> MKGTYLYLNIYKRKREASLITLNYIKNRFYPSKIQKIIKELFEDRLKGVEYDPNNANQLSE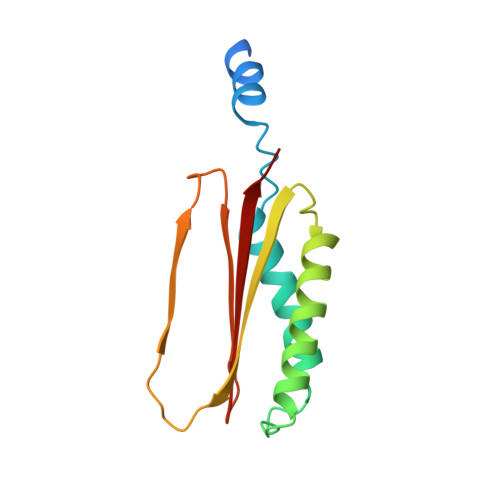RLVLELREKIKRGKVPRYKIGVQVVFGEIKGQGLRIASKCLWDVQNDNYASYTYTSEKVYCTGIVFGCYFE>[2x]MHHHHHHITSLYKKA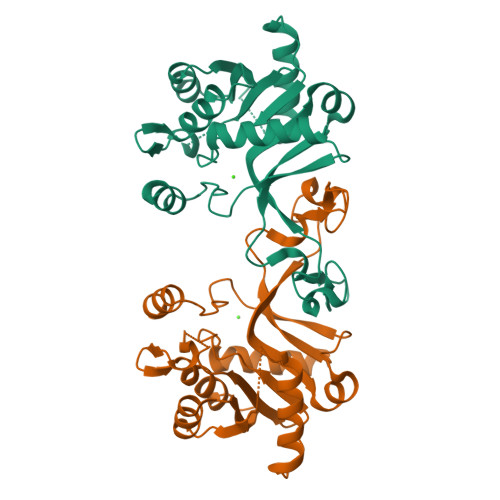GFMSNEYVALITARGGSKGLLRKNVLPLHGIPLIGWTIKAAQGCSYISKVFVSTDDYEIAKISEGLGALVINRPEELATDTASSIDVILHAISWLEQKEVQKYEGMILLQPTSPLRTSHHIKEAIELYEKTAAKFVISVFEPTHTPIKSYLENDDGTISGLYSNEAPYQRRQDLPRAYQPNGAIYAFSIDEFKLNNHFPRNKVFPYVMSEVESADIDTLEDLRKVEEQLKIKEINK> MTTYLEFIQQNEERDGVRFSWNVWPSSRLEATRMVVPVAALFTPLKERPDLPPIQYEPVLCSRTTCRAVLNPLCQVDYRAKLWACNFCYQRNQFPPSYAGISELNQPAELLPQFSSIEYVVLRGPQMPLIFLYVVDTCMEDEDLQALKESMQMSLSLLPPTALVGLITFGRMVQVHELGCEGISKSYVFRGTKDLSAKQLQEMLGLSKVPLTQATRGPQVQQPPPSNRFLQPVQKIDMNLTDLLGELQRDPWPVPQGKRPLRSSGVALSIAVGLLECTFPNTGARIMMFIGGPATQGPGMVVGDELKTPIRSWHDIDKDNAKYVKKGTKHFEALANRAATTGHVIDIYACALDQTGLLEMKCCPNLTGGYMVMGDSFNTSLFKQTFQRVFTKDMHGQFKMGFGGTLEIKTSREIKISGAIGPCVSLNSKGPCVSENEIGTGGTCQWKICGLSPTTTLAIYFEVVNQHNAPIPQGGRGAIQFVTQYQHSSGQRRIRVTTIARNWADAQTQIQNIAASFDQEAAAILMARLAIYRAETEEGPDVLRWLDRQLIRLCQKFGEYHKDDPSSFRFSETFSLYPQFMFHLRRSSFLQVFNNSPDESSYYRHHFMRQDLTQSLIMIQPILYAYSFSGPPEPVLLDSSSILADRILLMDTFFQILIYHGETIAQWRKSGYQDMPEYENFRHLLQAPVDDAQEILHSRFPMPRYIDTEHGGSQARFLLSKVNPSQTHNNMYAWGQESGAPILTDDVSLQVFMDHLKKLAVSSA;> EGL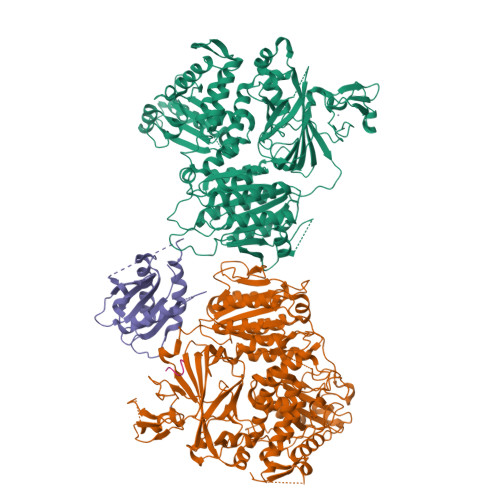RVVNLLQERNMLPSTPLKPPVPNLHEDIQKLNCNPELFRCTLTSIPQTQALLNKAKLPLGLLLHPFKDLVQLPVVTSSTIVRCRSCRTYINPFVSFLDQRRWKCNLCYRVNDVPEEFLYNPLTRVYGEPHRRPEVQNATIEFMAPSEYMLRPPQPPVYLFVFDVSHNAVETGYLNSVCQSLLDNLDLLPGNTRTKIGFITFDSTIHFYGLQESLSQPQMLIVSDIEDVFIPMPENLLVNLNESKELVQDLLKTLPQMFTKTLETQSALGPALQAAFKLMSPTGGRMSVFQTQLPTLGVGALKPREEPNHRSSAKDIHMTPSTDFYKKLALDCSGQQVAVDLFLLSGQYSDLASLGCISRYSAGSVYYYPSYHHQHNPVQVQKLQKELQRYLTRKIGFEAVMRIRCTKGLSIHTFHGNFFVRSTDLLSLPNVNPDAGYAVQMSVEESLTDTQLVSFQSALLYTSSKGERRIRVHTLCLPVVSTLNDVFLGADVQAISGLLANMAVDRSMTASLSDARDALVNAVIDSLSAYRSSVLSNQQPGLMVPFSLRLFPLFVLALLKQKSFQTGTNARLDERIFAMCQVKNQPLVYLMLTTHPSLYRVDNLSDEGALNISDRTIPQPPILQLSVEKLSRDGAFLMDAGSVLMLWVGKNCTQNFLSQVLGVQNYASIPQPMTDLPELDTPESARIIAFISWLREQRPFFPILYVIADESPMKANFLQNMIEDRTESALSYYEFLLHIQQQVNK;> MVLLTMIARVADGLPLAASMQEDEQSGRDLQQYQSQAKQLFRKLNEQSPTRCTLEAGAMTFHYIIEQGVCYLVLCEAAFPKKLAFAYLEDLHSEFDEQHGKKVPTVSRPYSFIEFDTFIQKTKKLYIDSRARRNLGSINTELQDVQRIMVANIEEVL;> GYSACEEEN>MREEEIRELYFKYFDENKLPFIQCNKCGHKFYYPRVLCPKCG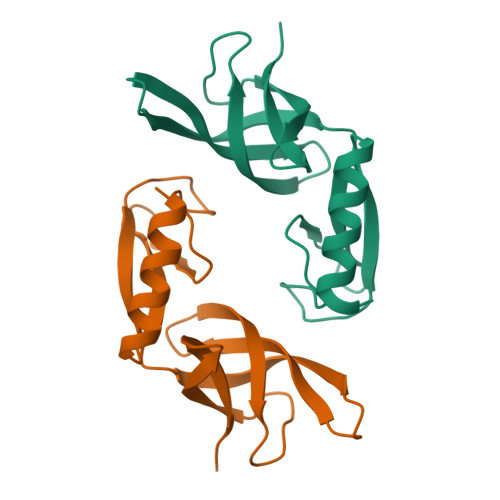SSDIEVRFSKGLGKIFAMTKVYRKDGSYVIYGIVELEEGFRMYSNIIEESQADINRKVEVIFKEINGKKYPLFKTVT[2x]1-(2-aminophenyl)-5-(trifluoromethyl)pyrazole-4-carboxylic acid | C11 H8 F3 N3 O2 | 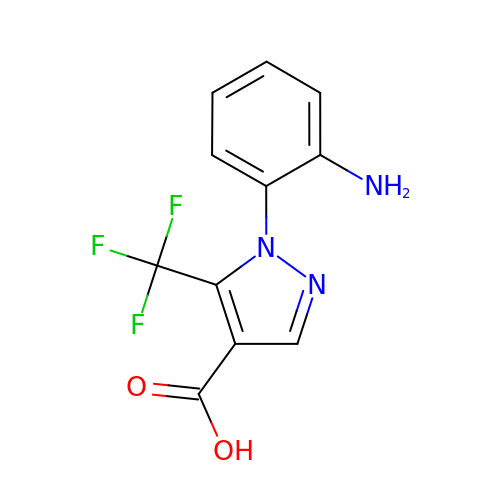NWURCYDONMHVOP-UHFFFAOYSA-N> RNILTNDEGLYAGQSLDVNPYHLIMQEDCNLVLYDHSTAVWSSNTDIPGKKGCKAVLQSDGNFVVYDAEGASLWASHSVRGNGNYVLVLQEDGNVV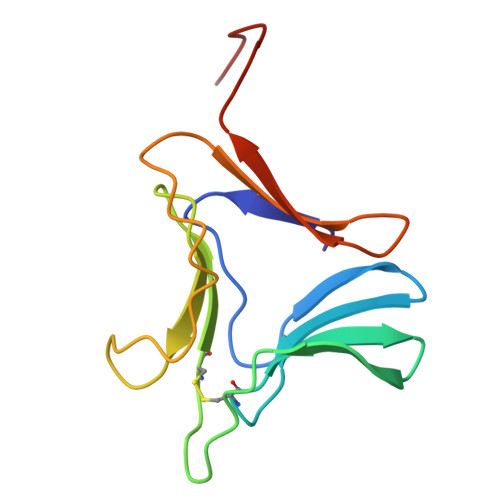IYGSDIWSTNTYK uridine-5'-diphosphate-3-O-(R-3-hydroxymyristoyl)-glucosamine 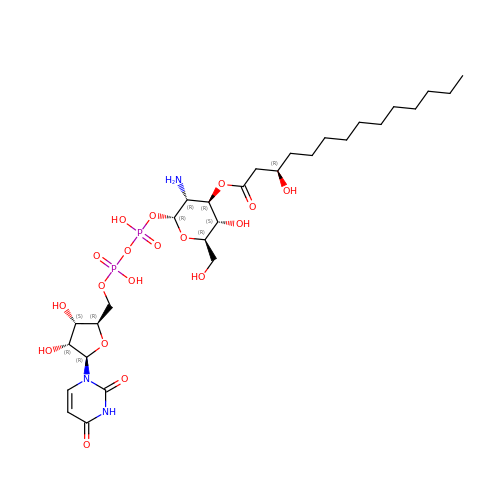| C29 H51 N3 O18 P2 | ZFPNNOXCEDQJQS-SSVOXRMNSA-N> ATVQQLEGRWRLVDSKGFDEYMKELGVGIALRKMGAMAKPDCIITCDGKNLTIKTESTL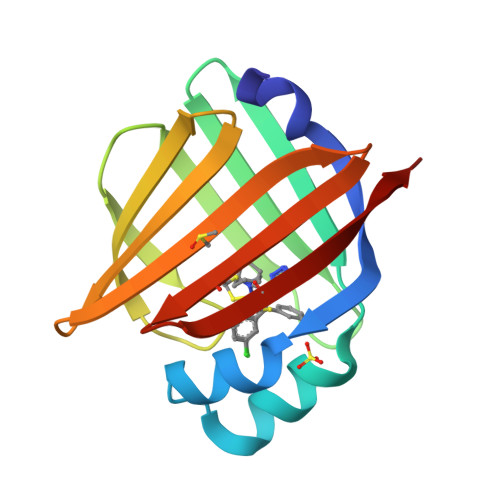KTTQFSCTLGEKFEETTADGRKTQTVCNFTDGALVQHQEWDGKESTITRKLKDGKLVVECVMNNVTCTRIYEKVE>[7x]EVKQENRLLNESESSSQGLLGYYFSDLNFQAPMVVTSSTTGDLSIPSSELENIPSENQYFQSAIWSGFIKVKKSDEYTFATSADNHVTMWVDDQEVINKASNSNKIRLEKGRLYQIKIQYQRENPTEKGLDFKLYWTDSQNKKEVISSDNLQLPELKQKSSNSRKKRSTSAGPTVPDRDNDGIPDSLEVEGYTVDVKNKRTFLSPWISNIHEKKGLTKYKSS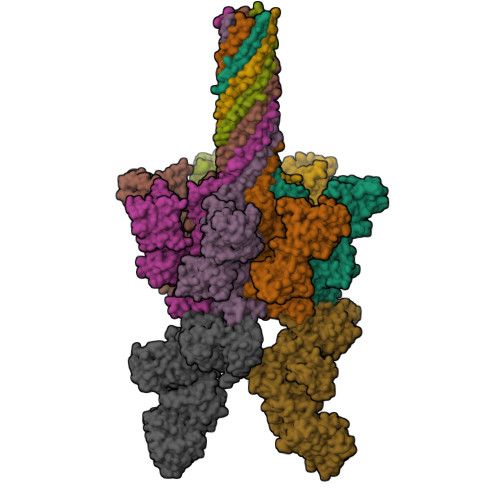PEKWSTASDPYSDFEKVTGRIDKNVSPEARHPLVAAYPIVHVDMENIILSKNEDQSTQNTDSQTRTISKNTSTSRTHTSEVHGNAEVHASFFDIGGSVSAGFSNSNSSTVAIDHSLSLAGERTWAETMGLNTADTARLNANIRYVNTGTAPIYNVLPTTSLVLGKNQTLATIKAKENQLSQILAPNNYYPSKNLAPIALNAQDDFSSTPITMNYNQFLELEKTKQLRLDTDQVYGNIATYNFENGRVRVDTGSNWSEVLPQIQETTARIIFNGKDLNLVERRIAAVNPSDPLETTKPDMTLKEALKIAFGFNEPNGNLQYQGKDITEFDFNFDQQTSQNIKNQLAELNATNIYTVLDKIKLNAKMNILIRDKRFHYDRNNIAVGADESVVKEAHREVINSSTEGLLLNIDKDIRKILSGYIVEIEDTEGLKEVINDRYDMLNISSLRQDGKTFIDFKKYNDKLPLYISNPNYKVNVYAVTKENTIINPSENGDTSTNGIKKILIFSKKGYEIG;>MNEHYTESDIKRNHKTEKNKTEKEKFKDSINNLVKTEFTNETLDKIQQTQDLLKKIPKDVLEIYSELGGEIYFTDIDLVEHKELQDLSEEEKNSMNSRGEKVPFASRFVFEKKRETPKLIINIKDYAINSEQSKEVYYEIGKGISLDIISKDKSLDPEFLNLIKSLSDDSDSSDLLFSQKFKEKLELNNKSIDINFIKENLTEFQHAFSLAFSYYFAPDHRTVLELYAPDMFEYMNKLEKGGFEKISESLKKEGVEKDRIDVLKGEKALKASGLVPEHADAFKKIARELNTYILFRPVNKLATNLIKSGVATKGLNVHGKSSDWGPVAGYIPFDQDLSKKHGQQLAVEKGNLENKKSITEHEGEIGKIPLKLDHLRIEELKENGIILKGKKEIDNGKKYYLLESNNQVYEFRISDENNEVQYKTKEGKITVLGEKFNWRNIEVMAKNVEGVLKPLTADYDLFALAPSLTEIKKQIPQKEWDKVVNTPNSLEKQKGVTNLLIKYGIERKPDSTKGTLSNWQKQMLDRLNEAVKYTGYTGGDVVNHGTEQDNEEFPEKDNEIFIINPEGEFILTKNWEMTGRFIEKNITGKDYLYYFNRSYNKIAPGNKAYIEWTDPITKAKINTIPTSAEFIKNLSSIRRSSNVGVYKDSGDKDEFAKKESVKKIAGYLSDYYNSANHIFSQEKKRKISIFRGIQAYNEIENVLKSKQIAPEYKNYFQYLKERITNQVQLLLTHQKSNIEFKLLYKQLNFTENETDNFEVFQKIIDEK[2x]>TNPVLDVDGNELQRGQLYYATSVMRPGGGLTLAAPKGSCPLNVAQAPFDEYSGRPLAFFPENADDDTVQEGSTLYIMFPEPTRCPQSTVWTFDREAGFVTTGGTTSKAIGPHNSRFAIRKAGDASSQPRDYQIEVCPCSTGVERPSCRMGCLGTLGLAEGGKNVLLNINNESPHTIRFVK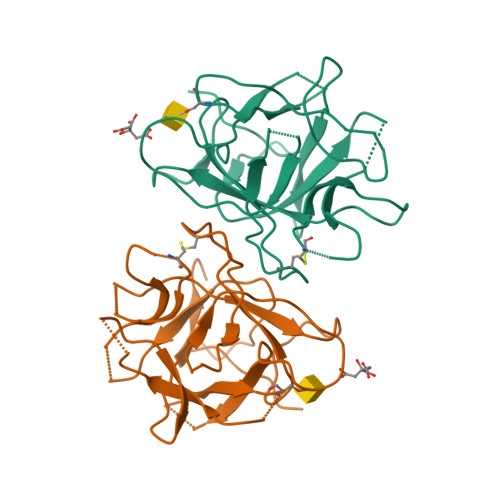VKEG[2x]>MKELVEMAVPENLVGAILGKGGKTLVE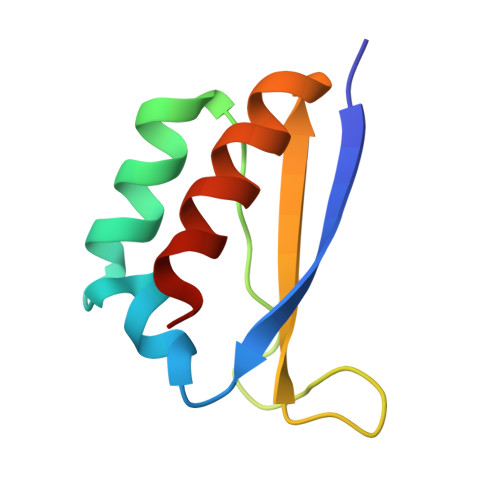YQELTGARIQISKKGEFLPGTRNRRVTITGSPAATQAAQYLISQRVTYE[4x]> DSARSFLERLEARGGREGAVLAGEFSDIQACSAAWKADGVCSTVAGSRPENVRKNRYKDVLPYDQTRVILSLLQEEGHSDYINGNFIRGVDGSLAYIATQGPLPHTLLDFWRLVWEFGVKVILMACREIENGRKRCERYWA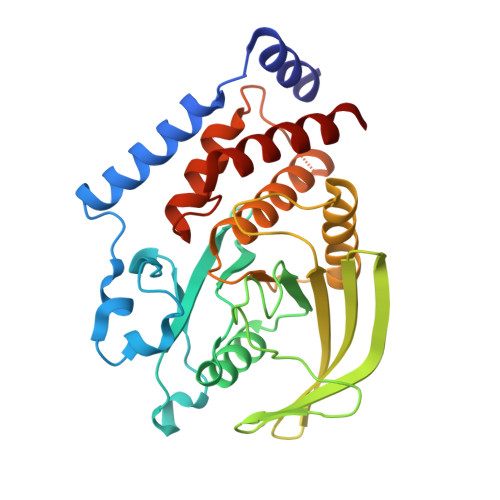QEQEPLQTGLFCITLIKEKWLNEDIMLRTLKVTFQKESRSVYQLQYMSWPDRGVPSSPDHMLAMVEEARRLQGSGPEPLCVHSSAGCGRTGVLCTVDYVRQLLLTQMIPPDFSLFDVVLKMRKQRPAAVQTEEQYRFLYHTVAQMFCST> MSYDVVIPAAGQGKRMKAGRNKLFIELKGDPVIIHTLRVFDSHRQCDKIILVINEQEREHFQQLLSDYPFQTSIELVAGGDERQHSVYKGLKAVKQEKIVLVHDGARPFIKHEQIDELIAEAEQTGAAILAVPVKDTIKRVQDLQVSETIERSSLWAVQTPQAFRLSLLMKAHAEAERKGFLGTDDASLVEQMEGGSVRVVEGSYTNIKLTTPDDLTSAEAIMESESGNKHV

The third enzyme is 2-C-Methyl-d-erythritol-4-phosphate cytidyltransferase (IspD), 4-diphosphocytidyl-2-C-methyl-d-erythritol (CDPME) is formed from MEP by reaction with CTP12. The subunit structure of BsIspD was of a compact α/β fold from which a long β-meander extended. The core of the enzyme consisted of a seven β-sheets (β2, β1, β4, β9, β5, β8, β10) where all strands were parallel, apart from β8 and β2. The β-meander lay between antiparallel strands β6 and β7 and made the major contribution to the dimer interface, and the lesser contribution came from the side-chain interactions of the residues on the α-helix fragment at the C-terminus.

Two crystal structures of BsIspD have been determined in orthorhombic crystal form with space group P212121 and P21212, named apo form I and II, respectively. In the apo form II, only one molecule (molecule C) was retained in the asymmetric unit, the functional dimer was formed by the sysmetry operation. Two flexible loop regions (residues 13–14, 226–232) were not built in the final model, because of the poor quality of the electron density. In the structure of apo form II, although the residues 13 and 14 were not built, it was clear that the P-loop shifted upward from the active site, since the Cα atoms of Gly11, Gln12 and Arg15 shifted 4.5 Å, 5.8 Å and 2.1 Å, respectively, meanwhile, the side chain of Arg15 flipped to extend to Asp81 which moved about 3 Å. Therefore, the active site was more exposed to the solvent than that in the apo form I. Moreover, the L1-loop also rotated about 30° and moved about 3.0 Å. Here the residues of Gly11 and Gln12 were too far to interact with residues at the same time, only one hydrogen bond was formed bewteen Arg15 and Asp81 (Arg15 NH1-Asp81 OD1 = 3.3 Å). The structural difference of the P-loop in the two apo forms may imply that the P-loop was quite flexible. The chain-to-chain superposition for 223 Cα positions revealed the r.m.s.d between subunits C-A and C-B were 0.41 Å and 0.46 Å, respectively, while the comparison on the dimer gave an r.m.s.d of 0.59 Å for 446 pairs of Cα atoms.>MDWVIPPISCPENEKGEFPKNLVQIKSNRDKETKVFYSITGQGADKPPVGVFIIERETGWLKVTQPLDREAIAKYILYSHAVSSNGEAVEDPMEIVITVTDQNDNRPEFTQEVFEGSVAEGAVPGTSVMKVSATDADDDVNTYNAAIAYTIVSQDPELPHKNMFTVNRDTG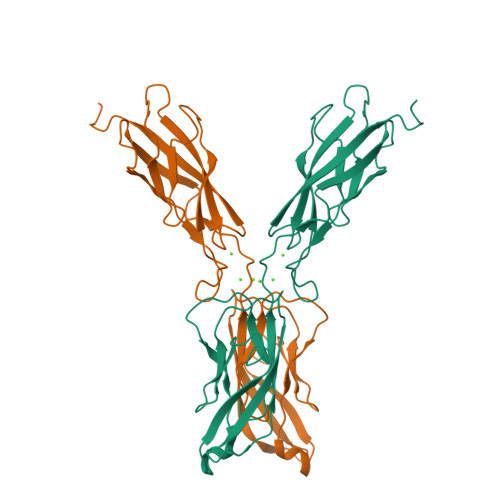VISVLTSGLDRESYPTYTLVVQAADLQGEGLSTTAKAVITVKDINDNA[2x]> MSRLDKSKVINSALELLNEVGIEGLTTRKLAQKLGVEQPTLYWHVKNKRALLDALAIEMLDRHHTHFSPLEGESWQDFLRNNAKSFRNALLSHRDGAKVHLGTRPTEKQYETLENQLAFLTQQGFSLENALYA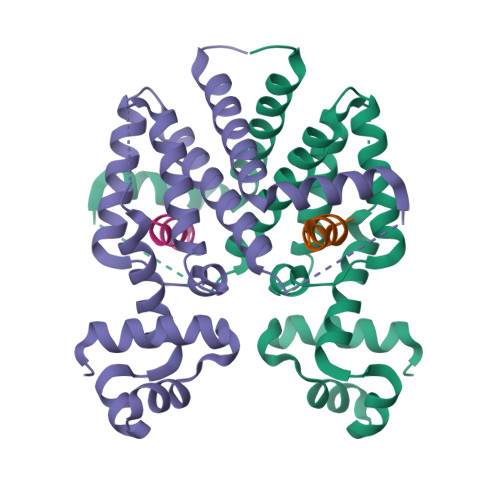LSAVGHFTLGSVLEDQEHQVAKEERETPTTDSMPPLLRQAIELFDHQGAEPAFLHGLESLIRGFEVQLTALLQIV;> KASEGLARVAALARSR>MPDMKLFAGNATPELAQRIANRLYTSLGDAAVGRFSDGEVSVQINENVRGGDIFIIQSTCAPTNDNLMELVVMVDALRRASAGRITAVIPYFGYARQDRRVRSARVPITAKVVADFLSSVGVDRVLTVDLHAEQIQGFFDVPVDNVFGSPILLEDMLQLNLDNPIVVSPDIGGVVRARAIAKLLNDTDMAIIDKRRPRANVSQVMHIIGDVAGRDCVLVDDMIDTGGTLCKAAEALKERGAKRVFAYATHPIFSGNAANNLRNSVIDEVVVCDTIPLSDEIKSLP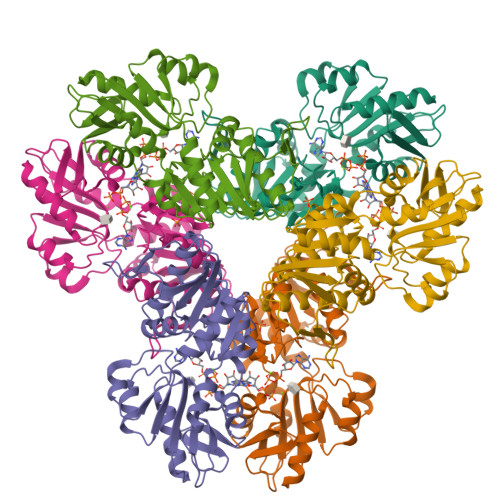NVRTLTLSGMLAEAIRRISNEESISAMFEHHHHHHH[6x]> GSHMASMKKKGSVVIVGRINLSGDTAYAQQTRGEEGCQETSQTGRDKNQVEGEVQIVSTATQTFLATSINGVLWTVYHGAGTRTIASPKGPVTQMYTNVDKDLVGWQAPQGSRSLTPCTCGSSDLYLVTRHADVIPVRRRGDSRGSLLSPRP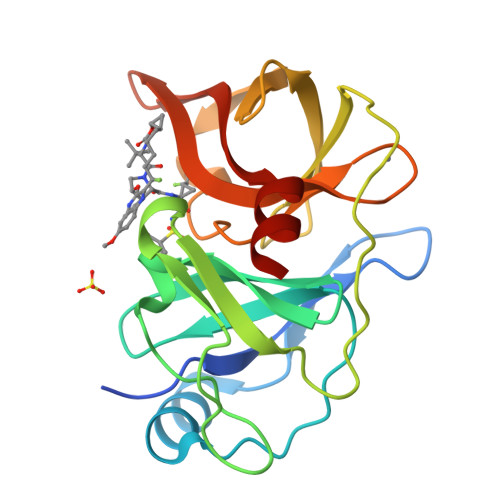ISYLKGSSGGPLLCPAGHAVGIFRAAVSTRGVAKAVQFIPVESLETTMRSP> NPKSLTRGPRDKPTPLEELLPHAIEFINQYYGSFKEAKIEEHLARLEAVTKEIETTGTYQLTLDELIFATKMAWRNAPRCIGRIQWSNLQ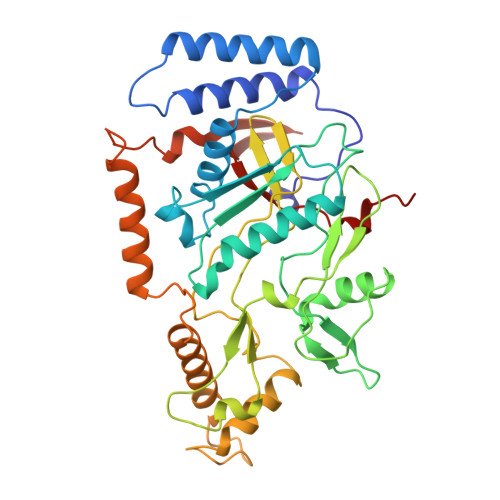VFDARNCSTAQEMFQHICRHILYATNNGNIRSAITVFPQRSDGKHDFRLWNSQLIRYAGYQMPDGTIRGDAATLEFTQLCIDLGWKPRYGRFDVLPLVLQADGQDPEVFEIPPDLVLEVTMEHPKYEWFQELGLKWYALPAVANMLLEVGGLEFPACPFNGWYMGTEIGVRDFCDTQRYNILEEVGRRMGLETHTLASLWKDRAVTEINVAVLHSFQKQNVTIMDHHTASESFMKHMQNEYRARGGCPADWIWLVPPVSGSITPVFHQEMLNYVLSPFYYYQIEPWKTHIWQNEHHHH>LPTAQEVQGLMARYIELV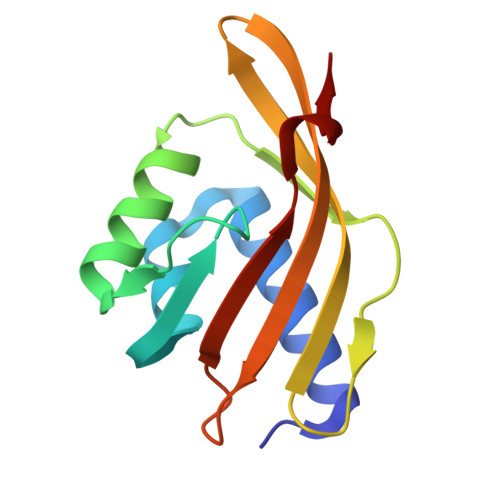DVGDIEAIVQMYADDATVEDPFGQPPIHGREQIAAFYRQGLGGGKVRACLTGPVRASHNGCGAMPFRIEMVWNGQPCAVDVIDVMRFDEHGRIQTMQAYWSEVNLSV[2x]> MVDTTKNTKLFTSYGVNTSKAVSPEMAAKIISKAKRPLLMVGTLALDPELLDRVVKISKAANIPIAATGSSLAVLADKDVDAKYINAHMLGFYLTDPKWPGLDGNGNYDMIITIGFKKFYINQVLSAAKNFSNL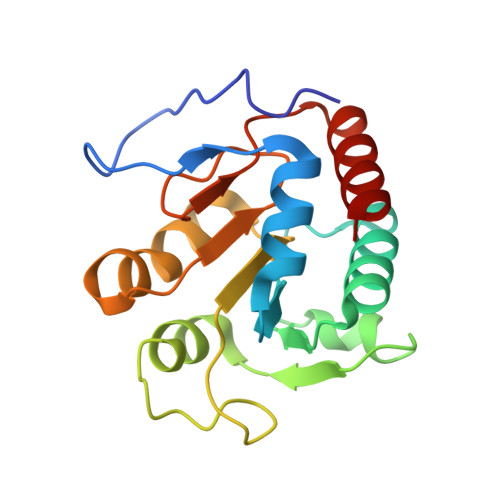KTIAIERGYIQNATMSFGNLSKADHYAALDELINAL> RSKSSNEATNITPKHNMKAFLDELKAENIKKFLYNFTQIPHLAGTEQNFQLAKQIQSQWKEFGLDSVELAHYDVLLSYPNKTHPNYISIINEDGNEIFNTSLFEPPPPGYENVSDIVPPFSAFSPQGMPEGDLVYVNYARTEDFFKLERDMKINCSGKIVIARYGKVFRGNKVKNAQLAGAKGVILYSDPADYFAPGVKSYPDGWNLPGGGVQRGNILNLNGAGDPLTPGYPANEYAYRRGIAEAVGLPSIPVHPIGYYDAQKLLEK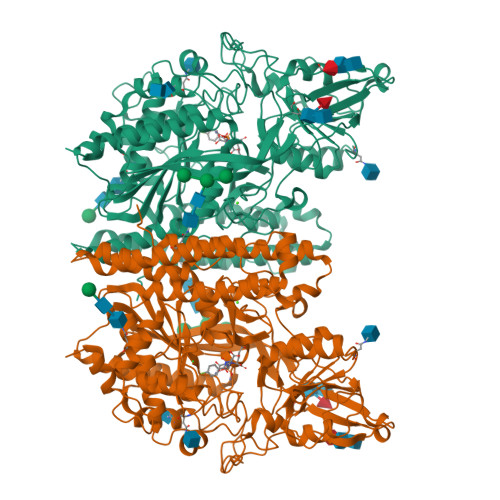MGGSAPPDSSWRGSLKVPYNVGPGFTGNFSTQKVKMHIHSTNEVTRIYNVIGTLRGAVEPDRYVILGGHRDSWVFGGIDPQSGAAVVHEIVRSFGTLKKEGWRPRRTILFASWDAEEFGLLGSTEWAEENSRLLQERGVAYINADSSIEGNYTLRVDCTPLMYSLVHNLTKELKSPDEGFEGKSLYESWTKKSPSPEFSGMPRISKLGSGNDFEVFFQRLGIASGRARYTKNWETNKFSGYPLYHSVYETYELVEKFYDPMFKYHLTVAQVRGGMVFELANSIVLPFDCRDYAVVLRKYADKIYSISMKHPQEMKTYSVSFDSLFSAVKNFTEIASKFSERLQDFDKSNPIVLRMMNDQLMFLERAFIDPLGLPDRPFYRHVIYAPSSHNKYAGESFPGIYDALFDIESKVDPSKAWGEVKRQIYVAAFTVQAAAETLSEVA>[4x]MSSEPPPPPQPPTHQASVGLLDTPRSRERSPSPLRGNVVPSPLPTRRTRTFSATVRASQGPVYKGVCKCFCRSKGHGFIT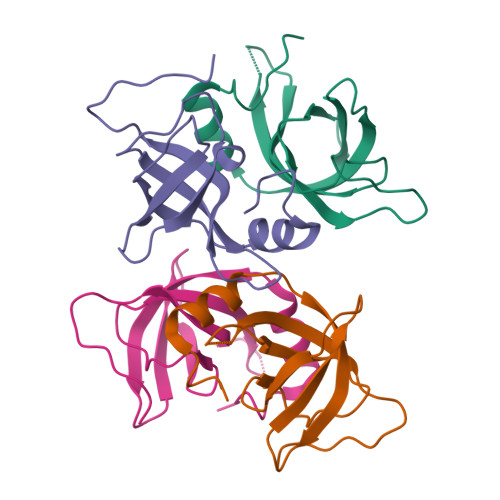PADGGPDIFLHISDVEGEYVPVEGDEVTYKMCSIPPKNEKLQAVEVVITHLAPGTKHETWSGHVISS>GSPEFTSQLVIMSELIELKQDGDLESLLEQHKNKLVVVDFFATWCGPCKTIAPLFKELSEKYDAIFVKVDVD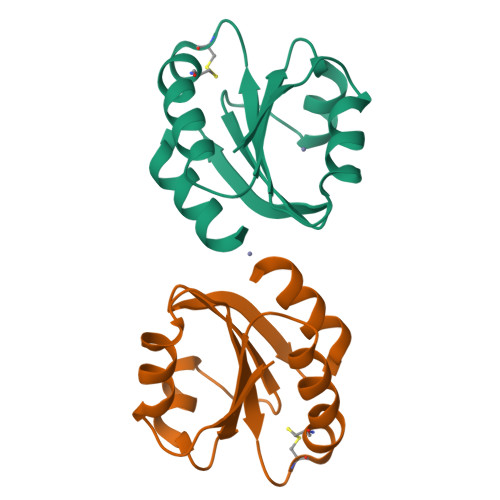KLEETARKYNISAMPTFIAIKNGEKVGDVVGASIAKVEDMIKKFI[2x]> MKIIKLYFESPVHFGEKRLSESKITFSADTLFSALMIEAVGLGKEDEFYQLASNNLVKFSDAFPFIDQYYYIPKPMFNLKLEKEDENPSKA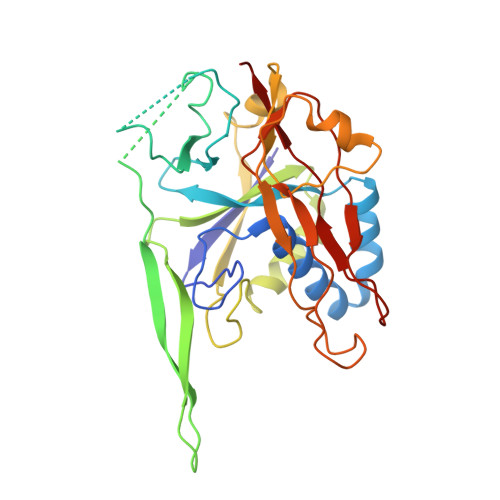FKKLLYVPIDSLEDYLSGGLDAYFERESFNLGKLALSEKVQQHDFKDSEPYNVGTFTFKENTGLYVLIEQTHPLLEELLENLQYSGIGGKRNSGYGKFKFEILEDSDIEDLFSAKGNRKILLSGALPKDAELEQALKNASYLLERRGGFVQSDTYATNLVKKQDLYVFKSGSTFENSFDGDIYQVGKKGNHPVYKYAKSFFLEVSV O-phosphono-N-(6-sulfanylhexanoyl)-L-threonine | C10 H20 N O7 P S | 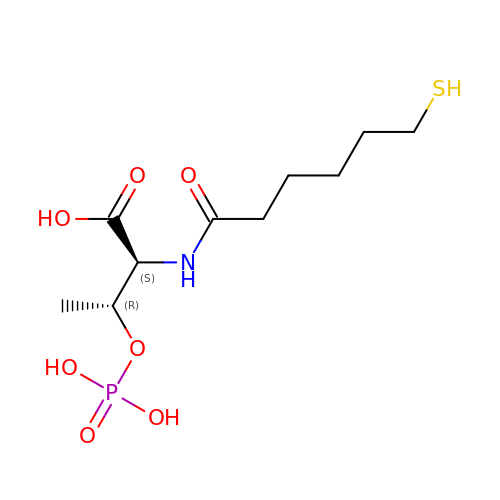PRNNQVAYHYUTOD-APPZFPTMSA-N> MPSLPTLQPLDLYRRTLACLVLAVSCLGGGGLWADDARTSIEQRSNAVSQVLLGIFSYVRWPKEPAVLQLSVVGPTEYADGLLRGMVQANGRRVHAERRAVDNPDLGTLCNVIYLGVVDERERQQVFRSLAGHPVLSISERGTECSVGSMFCLNVGGPRITFEANLDSIARSGVRVHPSVLKLARRQATP;> 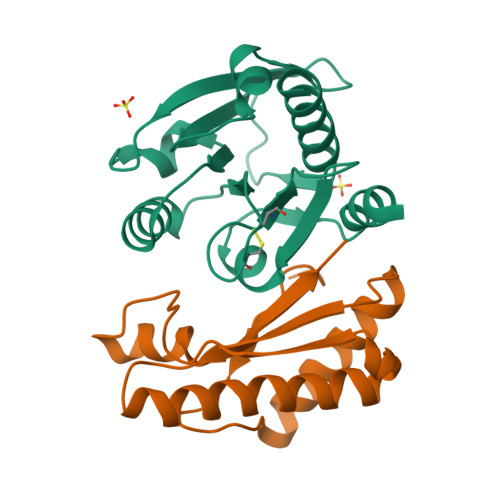MLPQRLHPSRLLALALFSLVLGLAGCQTKPPQTGLSAEQIAVLQEQGFELRDEGWPGSMSSKVLFGNNLDRLNPDSRNTLTKIARALLAVDIDKVRLEGHTDNYGDEGYNQKLSERRAESVAAVFREAGMPAANIEVRGLGMSKPVADNKTRAGRSENRRVAIIVPAE> MGSSHHHHHHHHLEVLFQGPHMEWIQSLPKIELHAHLNGSIRDST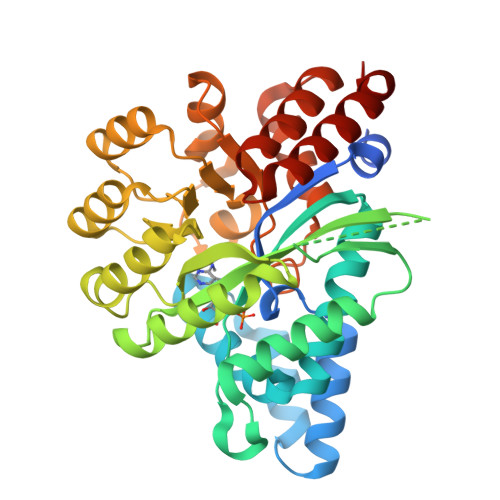LLELARVLGEKGVIVFADVEHVIQKNDRSLVEVFKLFDLIHKLTTDHKTVTRITREVVEDFALENVVYLELRTTPKRSDSIGMSKRSYMEAVIQGLRSVSEVDIDFVTASDSQKLHNAGDGIGRKKIYVRLLLSIDRRETTESAMETVKLALEMRDVGVVGIDLSGNPLVGEWSTFLPALQYAKDNDLHITLHCGEVPNPKEIQAMLDFKPHRIGHACFFKDEDWTKLKSFRIPVEICLTSNIVTKSISSIDIHHFADLYNAKHPLILCTNDFGVFSTSLSNEYALAVRSLGLSKSETFALARAAIDATFAEDEVKQQLRFIFDSASPEHV> VKLSHVEKDFIAFYSTTPHHLSYRDKTGGSYFITRLISCFRKHA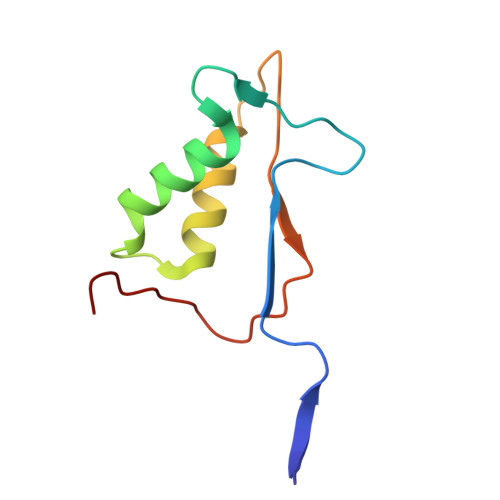CSCHLFDIFLKVQQSFEKASIHSQMPTIDRATLTRYFYLFPGN> GNSEEDYPNGTWLGDENNPEMRVRCAIIPSDMLHISTNCRTAEKMALTLLDYLFHREVQAVSNLSGQGKHGKKQLDPLTIYGIRCHLFYKFGITESDWYRIKQSIDSKCRTAWRRKQR

pmcThe BEN (BANP, E5R, and NAC1) domain is a ∼100-residue protein domain found in metazoans and viruses, but missing in nematodes and urochordates. There are nine BEN domain–containing transcription factors in the human genome, i.e., BANP, BEND2-7, and NAC1/2. The BEN domain-containing transcription factors regulate transcription by recruiting chromatin-modifying factors to specific chromatin regions via their DNA-binding BEN domains. Further structural analysis revealed that although all these BEN domains bind their target DNAs mainly through the insertion of the C-terminal α5 helix into the major groove of DNA, the residues of the α5 helices involved in the base interactions vary from one to another, explaining why they exhibit distinct DNA sequence preference.

We then carried out crystallization experiments and solved the structures of the BANP BEN domain in the apo form and in complex with the palindromic DNA by using the short and long constructs of the human BEN domain (aa 208-324 and aa 208-347), respectively. Structural analysis showed that the BEN domain of BANP mainly consisted of a short N-terminal β-hairpin, which was packed against a helix-bundle core of 5 α-helices. In the BANP-DNA complex structure, the extra C-terminal region after the helix α5 in the longer construct is disordered and unresolved in the structure. The structures of the BANP BEN domain in the apo form and the DNA complex overlaid very well with an RMSD of 0.68 Å over its 101 Cα atoms, suggesting that the DNA binding did not cause significant conformational changes. BANP also mediates the suppression of apoptotic genes BAX and PUMA through binding to their MARs elements during mild DNA damage, leading to cell cycle arrest. These findings suggest that BANP could bind to diverse DNA motifs, acting as either a transcription activator or a transcription repressor.>MDYKDDDDKEEGFRDRAAFIRGAKDIAKEVKKHAAKKVVKGLDRVQDEYSRRSYSRFEEEDDDDDFPAPSDGYYRGEGTQDEEEGGASSDATEGHDEDDEIYEGEYQGIPRAESGGKGERMADGAPLAGVRGGLSDGEGPPGGRGEAQRRKEREELAQQYEAILRECGHGRFQWTLYFVLGLALMADGVEVFVVGFVLPSAEKDMCLSDSNKGMLGLIVYLGMMVGAFLWGGLADRLGRRQCLLISLSVNSVFAFFSSFVQGYGTFLFCRLLSGVGIGGSIPIVFSYFSEFLAQEKRGEHLSWLCMFWMIGGVYAAAMAWAIIPHYGWSFQMGSAYQFHSWRVFVLVCAFPSVFAIGALTTQPESPRFFLENGKHDEAWMVLKQVHDTNMRAKGHPERVFSVTHIKTIHQEDELIEIQSDTGTWYQRWGVRALSLGGQVWGNFLSCFGPEYRRITLMMMGVWFTMSFSYYGLTVWFPDMIRHLQAVDYASRTKVFPGERVEHVTFNFTLENQIHRGGQYFNDKFIGLRLKSVSFEDSLFEECYFEDVTSSNTFFRNCTFINTVFYNTDLFEYKFVNSRLINSTFLHNKEGCPLDVTGTGEGAYMVYFVSFLGTLAVLPGNIVSALLMDKIGRLRMLAGSSVMSCVSCFFLSFGNSESAMIALLCLFGGVSIASWNALDVLTVELYPSDKRTTAFGFLNALCKLAAVLGISIFTSFVGITKAAPILFASAALALGSSLALKLPETRGQVLQ[2x]

Synaptic vesicle glycoprotein 2a (SV2A), a putative membrane transporter in the synaptic vesicles (SVs), has been identified as a target of LEV and BRV. SV2A also serves as a receptor for botulinum neurotoxin (BoNT), which is the most toxic protein and has paradoxically emerged as a potent reagent for therapeutic and cosmetic applications. SV2 family proteins belong to the major facilitator superfamily (MFS) with 12 predicted transmembrane helices. In addition to the transmembrane domain (TMD) core, a cytosolic N-terminal region and a large fourth luminal domain (LD4) are present.

We also determined the cryo-EM structure of the SV2A–LEV complex without HCA2 to a nominal resolution of 3.38 Å. SV2A forms a dimer, in which the two protomers are in an inverted configuration in the detergent micelle. Thus, the observed SV2A dimer is functionally irrelevant. The overall topologies of the SV2As are essentially the same in the presence and absence of HCA2. The cryo-EM density of LD4 is less resolved than that of TMD, suggesting a flexible movement of LD4 relative to TMD. This is further supported by the higher temperature B-factors of LD4 in the local resolution map.> ETGEVTLLDSRSVQGELGWIASPLEGGWEEVSIMDEKNTPIRTYQVCNVMEPSQNNWLRTDWITREGAQRVYIEIKFTLRDCNSLPGVMGTCKETFNLYYYESDNDKERFIRENQFVKIDTIAADESFTQVDIGDRIMKLNTEIRDVGPLSKKGFYLAFQDVGACIALVSVRVFYKRTKHHHHHH;> ETGSIVLEPIYWNSSNSKFLPGQGLVLYPQIGDKL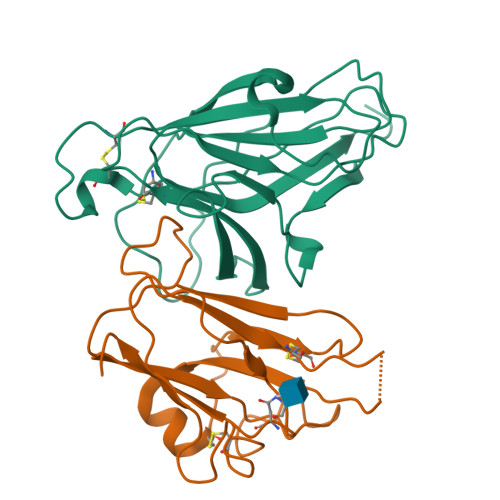DIICPKVDSKTVGQYEYYKVYMVDKDQADRCTIKKENTPLLNCAKPDQDIKFTIKFQEFSPNLWGLEFQKNKDYYIISTSNGSLEGLDNQEGGVCQTRAMKILMKVGQDGTKHHHHHH>GIGTGFPFDPHYVEVLGERMHYVDVGPRDGTPVLFLHGNPTSSYVWRNIIPHVAPTHRCIAPDLIGMGKSDKPDLGYFFDDHVRFMDAFIEALGLEEVVLVIHDWGSALGFHWAKRNPERVKGIAFMEFIR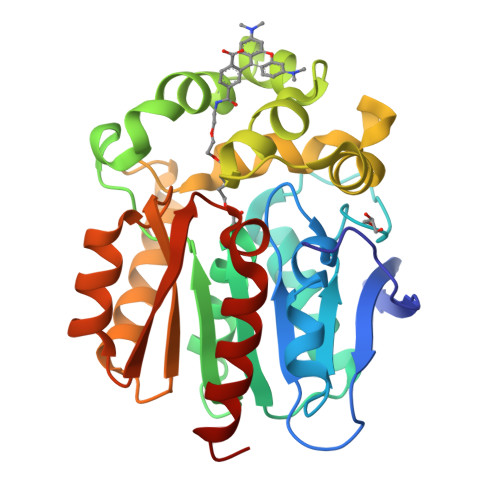PIPTWDEWPEFARETFQAFRTTDVGRKLIIDWNVFIEGTLPMGVVRPLTEVEMDHYREPFLNPVDREPLWRFPNELPIAGEPANIVALVEEYMDWLHQSPVPKLLFWGTPGVLIPPAEAARLAKSLPNCKAVDIGPGLNLLQEDNPDLIGSEIARWLSTLEI[6x]> MATPLAVNSAASLWGPYKDIWHKVGNALWRRQPEAVHLLDKILKKHKPDFISLFKNPPKNVQQHEKVQKASTEGVAIQGQQGTRLLPEQLIKEAFILSDLFDIGELAAVELLLAGEHQQPHFPGLTRGLVAVLLYWDGKRCIANSLKALIQSRRGKTWTLELSPELASMTTRFTDELMEQGLTYKVLTLVSQIDVNNEFEKLQRERGLGSEKHRKEVSDLIKECRQSLAESLFAWACQSPLGKEDTLLLIGHLERVTVEANGSLDAVNLALLMALLYCFDISFIEQSTEERDDMIHQLPLLTEKQYIATIHSRLQDSQLWKLPGLQATVRLAWALALRGISQLPDVTALAEFTEADEAMAELAIADNVFLFLMESVVVSEYFYQEEFYIRRVHNLITDFLALMPMKVKQLRNRADEDARMIHMSMQMGNEPPISLRRDLEHLMLLIGELYKKNPFHLELALEYWCPTEPLQTPTIMGSYLGVAHQRPPQRQVVLSKFVRQMGDLLPPTIYIPYLKMLQGLANGPQCAHYCFSLLKVNGSSHVENIQGAGGSPVSWEHFFHSLMLYHEHLRKDLPSADSVQYRHLPSRGITQKEQDGLIAFLQLTSTIITWSENARLALCEHPQWTPVVVILGLLQCSIPPVLKAELLKTLAAFGKSPEIAASLWQSLEYTQILQTVRIPSQRQAIGIEVELNEIESRCEEYPLTRAFCQLISTLVESSFPSNLGAGLRPPGFDPYLQFLRDSVFLRFRTRAYRRAAEKWEVAEVVLEVFYKLLRDYEPQLEDFVDQFVELQGEEIIAYKPPGFSLMYHLLNESPMLELALSLLEEGVKQLDTYAPFPGKKHLEKAVQHCLALLNLTLQKENLFMDLLRESQLALIVCPLEQLLQGINPRTKKADNVVNIARYLYHGNTNPELAFESAKILCCISCNSNIQIKLVGDFTHDQSISQKLMAGFVECLDCEDAEEFVRLEEGSELEKKLVAIRHETRIHILNLLITSLECNPPNLALYLLGFELKKPVSTTNLQDPGVLGCPRTCLHAILNILEKGTEGRTGPVAVRESPQLAELCYQVIYQLCACSDTSGPTMRYLRTSQDFLFSQLQYLPFSNKEYEISMLNQMSWLMKTASIELRVTSLNRQRSHTQRLLHLLLDDMPVKPYSDGEGGIEDENRSVSGFLHFDTATKVRRKILNILDSIDFSQEIPEPLQLDFFDRAQIEQVIANCEHKNLRGQTVCNVKLLHRVLVAEVNALQGMAAIGQRPLLMEEISTVLQYVVGRNKLLQCLHAKRHALESWRQLVEIILTACPQDLIQAEDRQLIIRDILQDVHDKILDDEAAQELMPVVAGAVFTLTAHLSQAVLTEQKETSVLGPAEAHYAFMLDSCFTSPPPEENPLVGFASIGDSSLYIILKKLLDFILKTGGGFQRVRTHLYGSLLYYLQIAQRPDEPDTLEAAKKTMWERLTAPEDVFSKLQRENIAIIESYGAALMEVVCRDACDGHEIGRMLALALLDRIVSVDKQQQWLLYLSNSGYLKVLVDSLVEDDRTLQSLLTPQPPLLKALYTYESKMAFLTRVAKIQQGALELLRSGVIVRLAQCQVYDMRPETDPQSMFGMRDPPMFIPTPVDRYRQILLPALQLCQVILTSSMAQHLQAAGQVLQFLISHSDTIQAILRCQDVSAGSLQELALLTGIISKAALPGILSELDVDVNEGSLMELQGHIGRFQRQCLGLLSRFGGSDRLRQFKFQDDNVEGDKVSKKDEIELAMQQICANVMEYCQSLMLQSSPTFQHAVCLFTPSLSETVNRDGPRQDTQAPVVPYWRLPGLGIIIYLLKQSANDFFSYYDSHRQSVSKLQNVEQLPPDEIK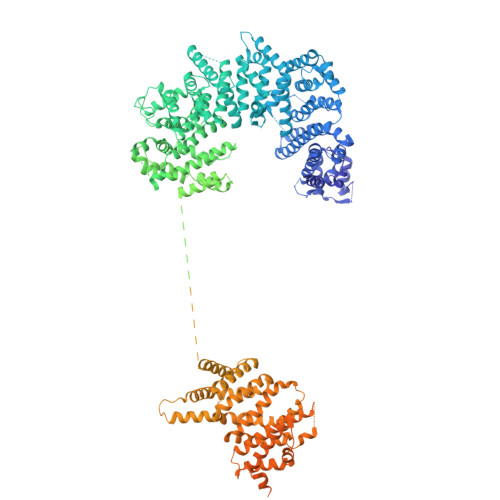ELCQSVMPAGVDKISTAQKYVLARRRLVKVINNRAKLLSLCSFIIETCLFILWRHLEYYLLHCMPTDSQDSLFASRTLFKSRRLQDSFASETNLDFRSGLAIVSQHDLDQLQADAINAFGESLQKKLLDIEGLYSKVRSRYSFIQALVRRIRGLLRISRN> AMRQCAIYGKGGIGKSTTTQNLVAALAEMGKKVMIVGCDPKADSTRLILHSKAQNTIMEMAAEAGTVEDLELEDVLKAGYGGVKCVESGGPEPGVGCAGRGVITAINFLEEEGAYEDDLDFVFYDVLGDVVCGGFAMPIRENKAQEIYIVCSGEMMAMYAANNISKG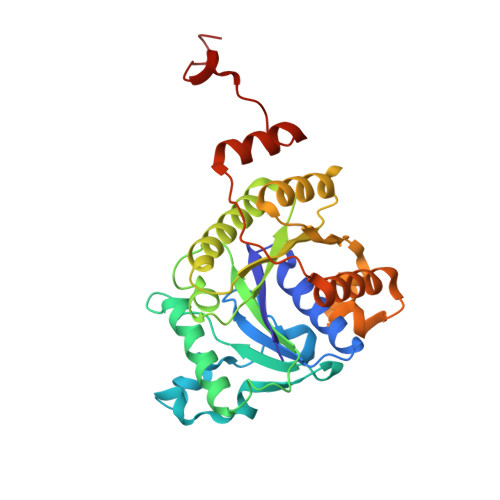IVKYANSGSVRLGGLICNSRNTDREDELIIALANKLGTQMIHFVPRDNVVQRAEIRRMTVIEYDPKAKQADEYRALARKVVDNKLLVIPNPITMDELEELLMEFGIMEVEDESIVGKTAEEV>MWKRSEQMKIKSGKCNMAAAMETEQLGVEIFETADCEENIESQDRPKLEPFYVERYSWSQLKKLLADTRKYHGYMMAKAPHDFMFVKRNDPDGPHSDRIYYLAMSGENRENTLFYSEIPKTINRAAVLMLSWKPLLDLFQATLDYGMYSREEELLRERKRIGTVGIASYDYHQGSGTFLFQAGSGIYHVKDGGPQGFTQQPLRPNLVETSCPNIRMDPKLCPADPDWIAFIHSNDIWISNIVTREERRLTYVHNELANMEEDARSAGVATFVLQEEFDRYSGYWWCPKAETTPSGGKILRILYEENDESEVEIIHVTSPMLETRRADSFRYPKTGTANPKVTFKMSEIMIDAEGRIIDVIDKELIQPFEILFEGVEYIARAGWTPEGKYAWSILLDRSQTRLQIVLISPELFIPVEDDVMERQRLIESVPDSVTPLIIYEETTDIWINIHDIFHVFPQSHEEEIEFIFASECKTGFRHLYKITSILKESKYKRSSGGLPAPSDFKCPIKEEIAITSGEWEVLGRHGSNIQVDEVRRLVYFEGTKDSPLEHHLYVVSYVNPGEVTRLTDRGYSHSCCISQHCDFFISKYSNQKNPHCVSLYKLSSPEDDPTCKTKEFWATILDSAGPLPDYTPPEIFSFESTTGFTLYGMLYKPHDLQPGKKYPTVLFIYGGPQVQLVNNRFKGVKYFRLNTLASLGYVVVVIDNRGSCHRGLKFEGAFKYKMGQIEIDDQVEGLQYLASRYDFIDLDRVGIHGWSYGGYLSLMALMQRSDIFRVAIAGAPVTLWIFYDTGYTERYMGHPDQNEQGYYLGSVAMQAEKFPSEPNRLLLLHGFLDENVHFAHTSILLSFLVRAGKPYDLQIYPQERHSIRVPESGEHYELHLLHYLQENLGSRIAALKVI[3x];>MP[3x]

Dipeptidyl peptidase 9 **(**DPP9) is a serine protease cleaving N-terminal dipeptides preferentially post-proline with (patho)physiological roles in the immune system and cancer. On the molecular level, proteases of the DPPIV family are serine aminopeptidases that remove dipeptides from the N-terminus of substrates having a Pro or an Ala residue in the second position (NH_2_-XaaPro/Ala). DPP8 and DPP9 are the only known intracellular members of this family, both localize to the cytosol, the nucleus and associate with the plasma membrane. Here we identify an association of human DPP9 with the tumour suppressor BRCA2, a key player in repair of DNA double-strand breaks that promotes the formation of RAD51 filaments.

Since DPP8 and DPP9 share a very similar substrate binding mechanisms *in vitro*, and since DPP9 crystals are notorious for being less well ordered, we also tested for a possible interaction between DPP8 and BRCA2. Similarly, in DPP8 all 3 copies of the asymmetric unit exhibit clearly interpretable electron density for the di-peptide. The well-ordered R-segment, a hallmark of ligand binding, was well defined and ordered and supports full occupation of the active sites. There was no trace of electron density for the rest of the peptide ([Fig fig2] and [Table tbl1]). (B) Shown is the N-terminal di-peptide of BRCA2 bound to both DPP9 and to DPP8. Omit map (Fo-Fc; 3σ) of a BRCA2 peptide soaked in DPP8 crystals (C222_1_) and in DPP9 crystals (P12_1_1). The R-Segment and SUBA are highlighted in orange and blue, respectively. For simplification, shown here is a monomer of DPP8.>MSLNITGIQSDWKVEKIEFAKLTGERARSAGANGRIGVHGKSCTVDIARITIDGQTGYGSSIHMTPEWAEDVIGRRLLDLFDDRGRLREAYRLQLEYPVLDWLGQRQGKPVYDLVSGAHLETGASLVVPCYDTSLYFDDLHLADERAAVALMQEEAMQGYAKGQRHFKIKVGRGGRHMPLWEGTKRDIAIVRGISEVAGPAGKIMIDANNAYNLNLTKEVLAALSDVNLYWLEAAFHEDEALYEDLKEWLGQRGQNVLIADGEGLASPHLIEWATRGRVDVLQYDIIWPGFTHWMELGEKLDAHGLRSAPHCYG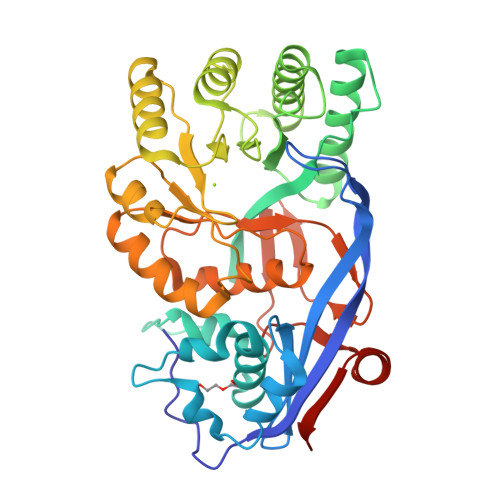NAYGIYASGHLSAAVRNFEFVEYDDITIEGMDVSGYRIENGEIHVPATPGFGIVFDDELVTYLINRSGWSEGHHHHHH[4x]>[14x]MIDVSSQRVNV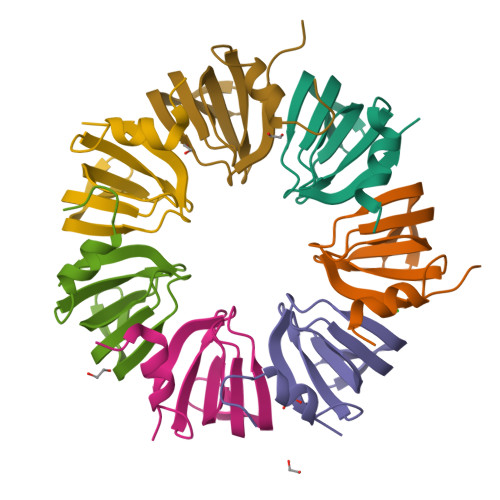QRPLDALGNSLNSPVIIKLKGDREFRGVLKSFDLHMNLVLNDAEELEDGEVTRRLGTVLIRGDNIVYISRGKLA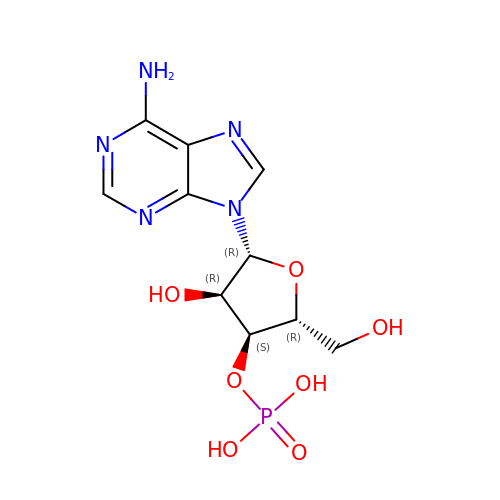[(2R,3S,4R,5R)-5-(6-aminopurin-9-yl)-4-hydroxy-2-(hydroxymethyl)oxolan-3-yl] dihydrogen phosphate | C10 H14 N5 O7 P | LNQVTSROQXJCDD-KQYNXXCUSA-N> MESGIDLQGQFISALQSLGLSHDLAKLLWLPLPMLMMLIVATVGVLVAVWLERKISAAVQQRIGPEYIGPLGILAPLADGLKLIFKEDVLPANSDRWLFTLGPAVVVIPVFLSYIIVPFGQNLLISNLAMGVFLWIALSSIAPIGLLMAGYASNNKYSLLGGLRAAAQSISYEIPLALAVLAVAMMSNGLGTVEIVEQQSQYGILSWNVWRQPIGFLVFWIAALAECERLPFDLPEAEEELVAGYQTEYAGMKFALFYLGAYVNLVLSALLVSVLYFGGWSFPIPLETIANLLGVSETNPFLQIAFAVLGITMTLIKAYFFVFLAILLRWTVPRVRIDQLLDLGWKFLLPVGLVNLLLTAGLKLAFPVAFGG;> MDLVTLAGQLNAGTILPETILIVTLLVVLLADLIQGRQADRWTPYFAIVGLGGAIATMIPLWTQPATISFFGSFISDHLSLFFRGLIALSALGTILMSIRYVEQTGSSLGEFMTILLTATVGGMFIAGAQELVFIFVALETLSIASYLLTGYTKRDSRSNEAALKYLLIGAASSAIFLYGSSLLYGLSGGHTQLPAIAQALSSESLGLVVALVFVIAGISFKISAVPFHQWTPDVYEGAPTPVVAFLSVGSKAAGFALAIRFLTLAFPSVTDQWQLIFTVLAILSMILGNVVALAQTSMKRMLAYSSIGQAGFVMIGFVVGTEAGYASMLFYLLVYLFMNLGAFTCVILFSLRTGTDQISEYAGLYQKDPLLTLGLSLCLLSLGGIPPLAGFFGKIYLFWAGWQAGAYGLVLLGLLTSVISIYYYIRVVKMMVVKEPQEMSEAVRNYPEVSWSSFGLRPLQVGLVMTVIATSLAGILANPLFNLVNTAVWDVPQLANQPTVMEVAYQALSPAGKS;> MVAIPRLRDTATVFVLSGYEYFLGFLIICSLVPVLALAASALLRPKSGRMIRLTTYESGMEPIGGAWIQFNVRYYMFALVFVIFDVETVFLYPWAVAFHQLGLLAFIEALIFIAILVVALVYAWRKRALEWS;> MLHSLRFLPMLTLLIVLPVIGALLMPLLPERVLRSVALVIAGLTFALSLWMLTQFDVHQSALQFTEFVPWLLPLGLNYSLGVDGLSLPLIVLGTFLTLGVVFTGEKTGQRLFYALVLLANAGITGALAAQNLLLFFLFYELELVPFYLLILIWGGQRREQAAVKFLIYTAVSGILVLAAFLAMGWLTHAPSFDSADIQIAGLAPTTQGILLLLLILGFGIKMPLVPLHSWLPDAYVEASTPTAILLGGALAKLGAYGLVRFALGYFPEAWAQFSGLLAIVAAVGIAYGALAAIAQKDIKRMVAYSSIGHMSYVLLAAAAHTHLSMVGAIAQMISHGLILALLFYLVGVIETKVGTRELNVLNGLLNPLRGLPTTSALLILGGMASAGIPGLVGFVAEFLIFQGSYGMFPLPTLVAVVGTGLTAVYFVIMINRTCFGRLDNRTAYYPRVVWSEKMPALVLTLLIVFLGVQPTWLVRWSETTSAQIVAAVPRTNELVATLAKR;> MQLTYVLILAALLFCIGIYGLVTSRNAVRVLMSIELLLNAVNLNLIGFANYLDGQQIKGQVFAVFVITVAAAEAAVGLAIILAIYRNRDTVDMEKFNLLKW;> MLQSFADTVWLIPFYSLAGMVLSLIWSPGITRKTGPRPAGYLNILLTFFSFVHALLATVAIANQPPQYLHWTWLDVAGLHLDIPVEISILTTTALMLITALNLMAQVFAVGYMEMDWGWARFFALLALFEGGMGALVLLDSLFFNYVVLEILTLATYLLIGLWFNQPLVVTGARDAFLTKRVGDLVLLMGVLAIYPLAGSWNYDDLAAWAATAQVNSTLITLICLALIAGPMGKCAQFPLHLWLDEAMEGPIPASILRNAVVVATGAWVLVKLTPVLSLSPVALTALLVIGSVTALGGTLIAIAQVDIKRALSYLVSAYMGWVFIAVGLKEPGLAFVFILTYSLAMAVLMMSIGSIIWNSVTQDLRLLGGLWSRRPISGISFLVGSAGLLAVPPLASFFPQAELLDTAFAQLPWVGGVLLLMNTFAAFSLGRTFCLVWGGEVKPMTARSPEVFWPMILPMTVDLGLVLHLPILMARFDWVIWTQPSLATAAALTITALLGWGVAAWVYLGKAIPKPVQFPLPSVQNLLAYDFYTPKLYRATVVGVVDMISRITAWFDRTFVDGTGNAFGVVTLLGGDR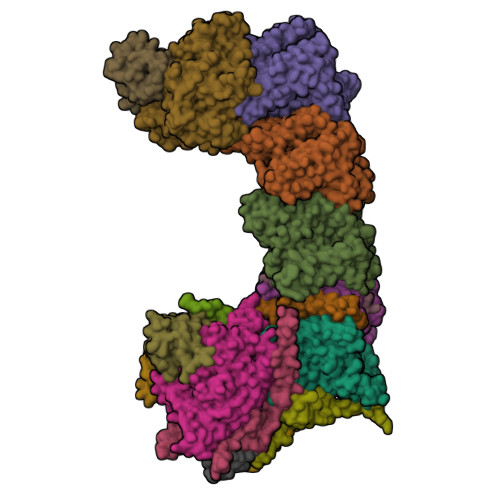LKYSTTGQSQAYILTILMGIAILVIAICWPLLA;> MDLATLTQTITFFALAAAVIIAALGVVLLDNVVYSAFLLGGVFLSIAGLYILMNADFVSAAQILIYVGAVNVLILFAIMLVNKRETYTPVPGRWLRQGGAAVVSLGVFALLTKMILQTPWQLSSVPPTPDSITTIGQHFFSDFLLPFELASVLLLMALIGAVVLARRELVLEPEPILGEEVVPPLELPERPREPVALSEK;> MPKIETRTEPMVINMGPHHPSMHGVLRLMVTLDGEDVIDCEPVIGYLHRGMEKIAENRTNIMFIPYVSRWDYAAGMFNEAVTVNAPEKLAGIPVPKRASYIRVIMLELNRIANHLLWLGPFLADVGAQTPFFYIFREREYIYDLFEAATGMRFINNNYFRIGGVAADLTYGWVTKCRDFCDYFLPKVDEYERLITNNPIFVRRLQGVGKISREEAINWGLSGPMLRASGVKWDLRKVDHYECYDDFDWDVPVATEGDCLARYIVRIQEMRESVKIIRQALDGLPGGPYENLEAKRMLEGAKSEWNGFDYQYIGKKLSPTFKIPKGEHYVRVESGKGELGIYLIGDDNVFPWRWKIRPPDFNNLQVLPQLLKGMKVADIVAILGSIDVIMGSVDR;> MKFLNQITNYAKEAVQSAKYIGQGLSVTFDHMRRRPITVQYPYEKLIPSERFRGRIHFEFDKCIACEVCVRVCPINLPVVDWVFNKELKKKELKHYSIDFGVCIFCANCVEYCPTNCLSVTEEYELATYDRHELNYDSVAMGRIPYKVTQDPMVTPIREFAYLPAGVMSGHDLPAGAQRAGERPEAIANTAKSSEN;> MSDTPEAPIVEAGPVGRLLQSQNLSVESLGRDASGVEMIKVDRDRLLAVCQTLYADGFNYLRCQAAYDSGPGQDLVSTYHLIKLSDNADRPPEVRIKVFVPRDDPRVPSVYWIWKTADWQERESYDMFGIVYEGHPNLKRILMPEDWVGWPLRKDYITPDFYELQEAY;> MTNTTSPAILNPIARPEVPQELAENIILTSLNDVYDWARLSSLWPLMYGTACCFIEFAAMIGSRFDFDRFGLVPRNSPRQADLIITSGTITMKMAPALVRLYEQMPSPKYVIAMGACTITGGMFSSDSYSAVRGVDKLIPVDVYLPGCPPRPEAIMDAIVKLRKKIANEHINERGNLAQTHRLFTAKHKMKPVPPILTGQYLNAPSRQAPPPALAAAMGIAVPALGEAVSETTSVAE;> MAVSTELLVLGVYGALAGLYLLVVPAIVYAYLNARWYVASSFERAFMYFLVTFFFPGLLLLAPFINFRPQPRSLNS;> MLLKSTTRHVHIYAGHVVDGEVHPDTETLTLNVDPDNELEWNEAALAKVEAKFRELVANAAGEDLTEYNLRRIGSDLEHFIRSLLMQGEIGYNLNSRVRNYSLGIPRVNHS;> MGLLAGYQFVKDLESAGALALFVPPEGGFEGRYQRRLRSKGYTTLPMSAPGLGDLAAYLTQEHGIRPAHTGKEDIRVYFQPPLVTYHLENLPPNAKGLVLWLIDGKRLSKQEFAYLAQLTQTLPKFKVVVEVGGDRVVRWEPLADWVAAA;> MAIKKGDLVKVVAEKLANSLEALASDHRYPPYLFEGRGEVVDIRGDYAQIKFPVPTPTVWLRLDQLEVAQ;> MVQAMERPSSAKLPPLDHPLADIIYRLEAGGALIPDTPVNLMKIIGMYKAYSIPMDFYWRDLLYLGERVFINPFPFFKYFPTKEYFELPNHYAGDTADLRIWRGPAHAHPELMEFIEKGETGKMPRLLHHLWHDRINMEFSEDLARAMMWHRMGGQLDIYLDSEEYKAAADKAIRAYFKRNPLMLGLYKLFPDLFLEQARQATYMNVLGLFWEVMAPVFFEISDRYDEGSITSVKDAMNFLVNGIFAIAGRPIYHHVYIDDEVHVLVPKEKGFMWLYEAAFPYVEAVFYRTSPFRGTKSYNAQANQVPTDQVDFHYGILFADKFPVGTAGIPPTLLHQDMYHFLPQYLKDYFHQHCRGEDDILVQLGIAFQHAMYTVTSAVLQATRAAFYYPLDDPNPEHLMANRRFFVAQMDRFLRPQYGIAEACKIRNVQDPNYL;> MATIVDIAVNTPGFSTLVTAVKVANLVEALQSPGPFTVFAPNDDAFAKLPDGTITSLVQNPPQLGRILKYHVVAGAYKATDLKRMGIVTSLEGSTIPIHGDNPLEVKNATVLAADIEAENGIIHVIDTVILMGLDPAHSFQETNIPYKV;> MIRPIADTYPLLPLSKAQMGQRQEIINSHKRLWDKTMATDLIMTILPGMTVKVTNPNDTYYQFQGIVQRITDGKVAVLFEGGNWDKLVTFQASELEPVVVTPKEKAKAKK2*-DEOXY-THYMIDINE-5*-ALPHA BORANO DIPHOSPHATE (ISOMER RP) | C10 H19 B 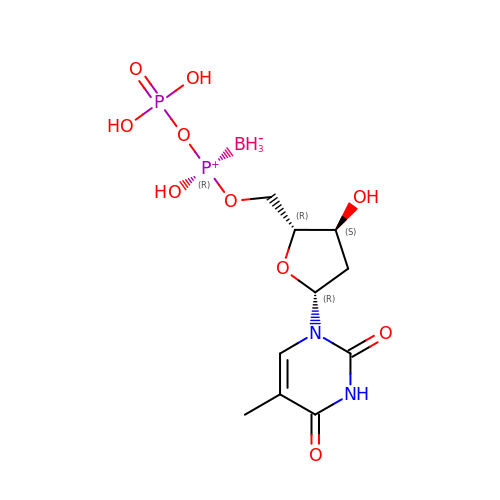N2 O10 P2 | QDZZFSSDQOLCBV-TYNZIUOXSA-N>MAELPPGRLATTEDYFAQQAKQAVTPDVMAQLAYMNYIDFISPFYSRGCSFEAWELKHTPQRVIKYSIAFYAYGLASVALIDPKLRALAGHDLDIAVSKMKCKRVWTDWEEDGFGTDPIEKENIMYKGHLNLMYGLYQLVTGSRRYEAEHAHLTRIIHDEIAANPFAGIVCEPDNYFVQCNSVAYLSLWVYDRLHGTDYRAATRAWLDFIQKDLIDPERGAFYLSYHPESGAVKPWISAYTTAWTLAMVHGMDPAFSERYYPRFKQTFVEVYDEGRKARVRETAGTDDADGGVGLASAFTLLLAREMGDQQLFDQLLNHLEPPAKPSIVSASLRYEHPGSLLFDELLFLAKVHAGFGALLRMPPPA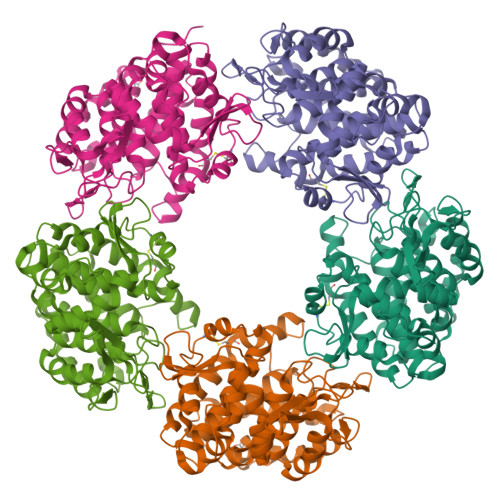AKLAGK[5x]> MKDIAIRGYCDRPSVATGETIRFYVSANETRGTFDAELVRLIHGDSNPAGPGYKEEAIKSDLEGQYPARFQRTQFGSYVEVADPDAGLQPDGAFSVHLFLWSTTPSRGRQGIASRWNDERQSGWNLAIEDGRVVFTIGDGSGATSSVVSDRPLFQQIWYSITGVYDPEKKQLRLYQKSVVNRTNSRFGLVVPLDSDCAVSADATVKAADSETSLLIAGLGEAAAQDGRTWCIAHYNGKVDAPKIYGCALGQDDAEKLSRGEIVRPISRLAHWDFSAGIGLNGIPTDHVVDASGYGHHGRCMNQPSRGSTGWNWDGHEENFIHCPEQYGALWFHEDCLDDCRWEKDFEFTVPEGLKSDFYAVKIRYEDTEDYIPFFVLPPRGTATAPILVIASTLSYLAYANEQIMHKADIGQAVAGHTPVLNEN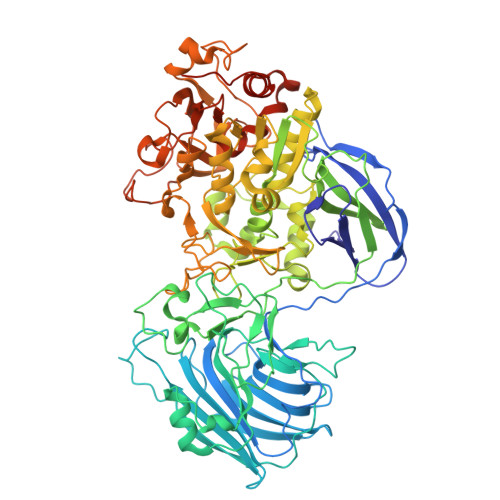DVELHKNLSYYGLSTYDGHIDGRGVQYTSWRRPIMNLRPKHRQGFGSIWELPADLHLIDWLNHNGFEYDVATEHDLNDQGAELLRRYKVVLTGSHPEYQTWANADAWEDYLADGGRGMYLAANGMYWIVEVHPEKPWVMEVRKELGVTAWEAPPGEYHYSTNGRRGGRFRGRARATQKIWGTGMSSFGFDHSGYFVQMPDSQDERVAWIMEGIDPEERIGDGGLVGGGAGGYELDRYDLALGTPPNTLLLASSVEHSVVYTVIPDDKAFPHPGMNGGEHPFVRADITYFSTANGGGMFATSSISWLGSLSWNDYDNNVSKMTKNVLNQFIKDEPAPRVKLAAALEHHHHHH4-METHYL-3-({3-[2-(METHYLAMINO)PYRIMIDIN-4-YL]PYRIDIN-2-YL}OXY)-N-[2-MORPHOLIN-4-YL-5-(TRIFLUOROMETHYL)PHENYL]BENZAMIDE | C29 H27 F3 N6 O3 | 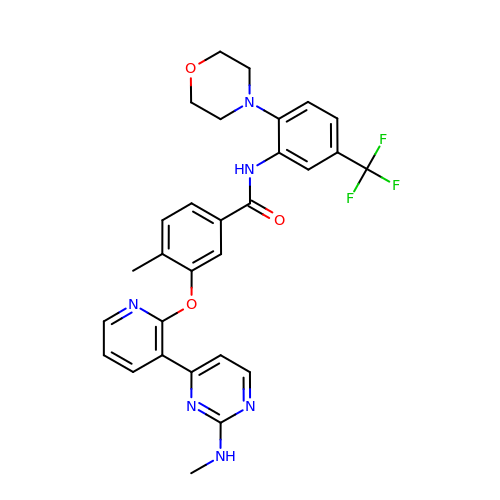HHKWHHAJTWLRKG-UHFFFAOYSA-N> PANKMSMSTMNMPMAMKVGGGGSGGGGSGGGGSSAFFFCGAISECHYLNGTERVRYLQRYIYNRQQYAHFDSDVGKFVADSPLGEPQAEYWNSNAELLENRMNEVDRFCRHNYGGVESFTVQRSVEPKVRVSALQSGSLPETDRLACYVTGFYPPEIEVKWFLNGREETERVVSTDVM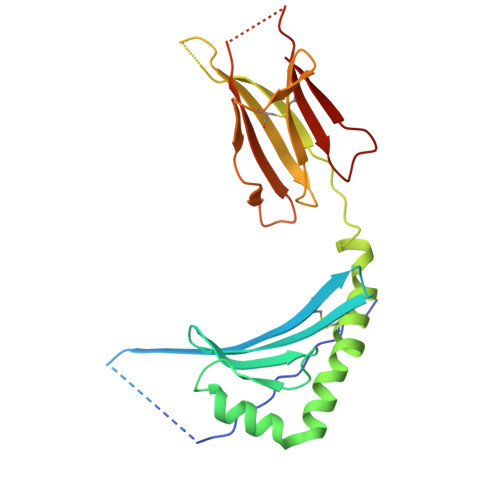QNGDWTYQVLVVLETVPRRGDSYVCRVEHASLRQPISQAWE>MNITIYDVAREANVSMATVSRVVNGNPNVKPTTRKKVLEAIERLGYRPNAVARGLASKKTTTVGVIIPDISSIFYSELARGIEDIATMYKYNIILSNSDQNMEKELHLLNTMLGKQVDGIVFMGGNITDEHVAEFKRSPVPIVLAASVEEQEETPSVAIDYEQAIYDAVKLLVDKGHTDIAFVSGPMAEPINRSKKLQGYKRALEEANLPFNEQFVAEGDYTYDSGLEALQHLMSLDKKPTAILSATDEMALGIIHAAQDQGLSIPEDLDIIGFDNTRLSLMVRPQLSTVVQPTYDIGAVAMRLLTKLMNKEPVEEHIVELPHRIELRKSTKSHHHHHH[2x];>[2x]AQKTFKVTADSGIHARPATVLVQTASKYDAD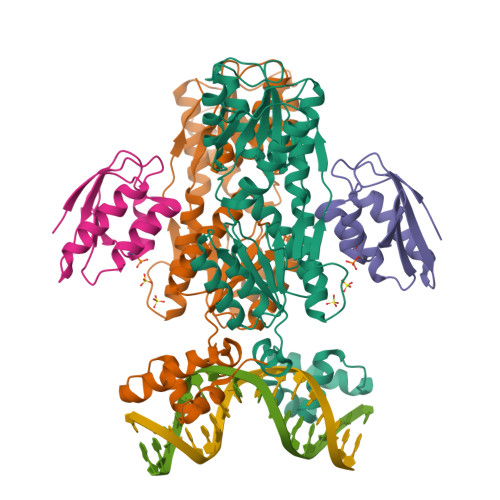VNLEYNGKTVNLKSIMGVMSLGIAKGAEITISASGADENDALNALEETMKSEGLGE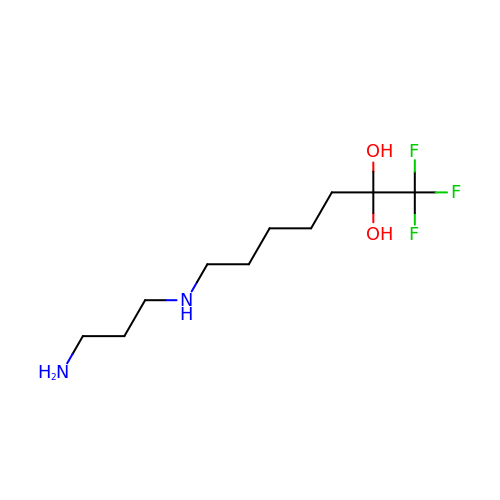7-[(3-aminopropyl)amino]-1,1,1-trifluoroheptane-2,2-diol | C10 H21 F3 N2 O2 | IVRAKANOVJJYCX-UHFFFAOYSA-N> MVNNNRPRRQRAQRVVVTTTQTAPVPQQNVPRNGRRRRNRTRRNRRRVRGMNMAALTRLSQPGLAFLKCAFAPPDFNTDPGKGIPDRFEGKVVSRKDVLNQSISFT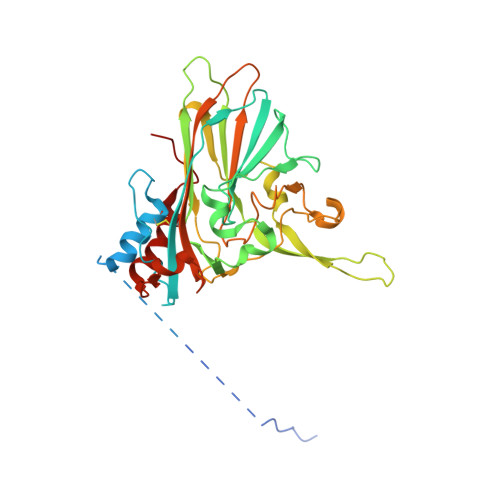AGQDTFILIAPTPGVAYWSASVPAGTFPTSATTFNPVNYPGFTSMFGTTSTSRSNQVSSFRYASMNVGIYPTSNLMQFAGSITVWKCPVKLSTVQFPVATDPATSSLVHTLVGLNGVLAVGPDNFSESFIKGVFSQSACNEPNFQFNDILQGIQTLPPANVSLGSTGQPFTMDSGAEATSGVVGWGNMDTIVIRVSAPEGAVNSAILKAWSCIEYRPNPNAMLYQFGHDSPPLDEVALQEYRTVARSLPVAVIAAQN> MQDAITSVINSSDVQGKYLDNAALEKLKGYFATGELRVRAATTISANAAAIVKEAVAKSLLYSDITRPGGNMYTTRRYAA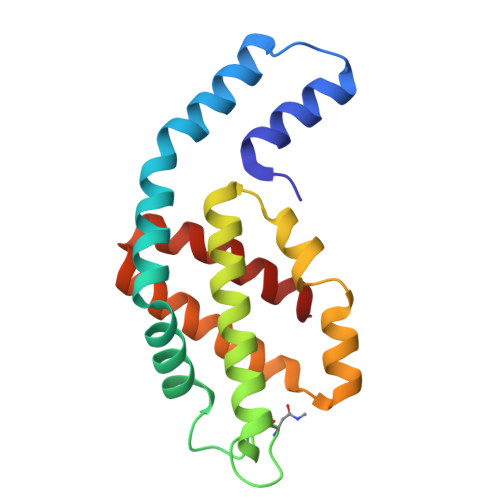CIRDLDYYLRYATYAMLAGDPSILDERVLNGLKETYNSLGVPVGATVQAIQAIKEVTASLVGPDAGKEMGVYFDYICSGLS>MTQMSDEQFRIFIETIKSLGPIKEEPPSKGSFSNCTVRFSGQRDHDAVDEFINAVETYKEVEGISDKDALKGLPLLFKSIAVVWWKGVRRDAKTWSDALQLLRDHFSPTKPSYQIYMEIFETKQSYDEVIDSFICKQRALLAKLPEGRHDEETELDFIYGLMQPKYRESIPRHEVKT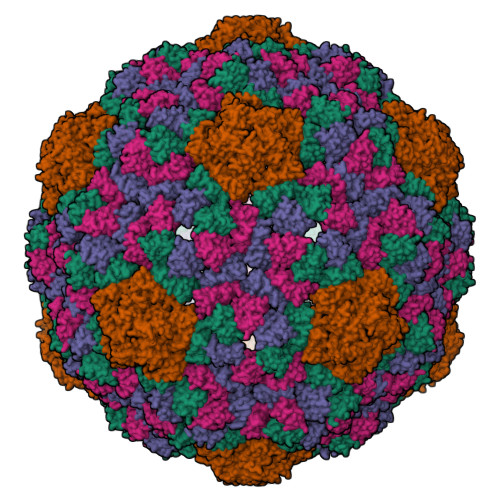FRELLDRGRTVERTRH[4x]> DFPNNKETGEALLTPVDATASSHDGNGPDRLID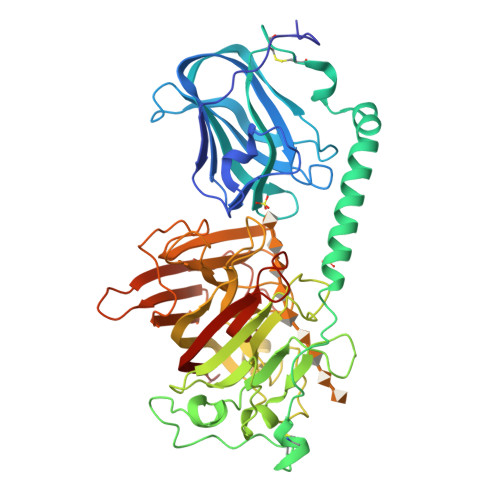QDLTTRWSSAGDGEWAMLDYGSVQEFDAVQASFSKGNERQSKFDIQVSVDGETWTTVLENQLSSGKAIGLERFQFEPAVKARYVRYVGHGNTKNGWNSVTGLAAVNCSINACPASQIITSDVVAAEAVLIAEMKAAEKARKAARKDLRSGNFGVAAVYPCETSVKCDTRSALPVPTGLPATPVAGNAPSENFDMTHWYLSQPFDHDKNGKPDDVSEWNLANGYQHPEIFYTADDGGLVFKSYVKGVRTSKNTKYARTELREMMRRGDQSISTKGVNKNNWVFSSAPEADLEAAAGIDGVLEATLKIDHATTTGNANEVGRFIIGQIADQNDEPIRLYYRKLPNQPTGAVYFAHESQDATKEDFYPLVGDMTAEVGEDGIALGEVFSYRIDVKGNTMTVTLMREGKDDVVQVVDMSNSGYDVGGKYMYFKAGVANQNISGDLDDYSQATFYQLDVSHDQYKK>[4x]ADPKCTVSHEVADCSHLKLTQVPDDLPTNITVLNLTHNQLRRLPAANFTRYSQLTSLDVGFNTISKLEPELCQKLPMLKVLNLQHNELSQLSDKTFAFCTNLTELHLMSNSIQKIKNNPFVKQKNLITLDLSHNGLSSTKLGTQVQLENLQELLLSNNKIQALKSEELDIFANSSLKKLELSSNQIKEFSPGCFHAIGRLFGLFLNNVQLGPSLTEKLCLELANTSIRNLSLSNSQLSTTSNTTFLGLKWTNLTMLDLSYNNLNVVGNDSFAWLPQLEYFFLEYNNIQHLFSHSLHGLFNVRYLNLKRSFTKQSISLASLPKIDDFSFQWLKCLEHLNMEDNDIPGIKSNMFTGLINLKYLSLSNSFTSLRTLTNETFVSLAHSPLHILNLTKNKISKIESDAFSWLGHLEVLDLGLNEIGQELTGQEWRGLENIFEIYLSYNKYLQLTRNSFALVPSLQRLMLRRVALKNVD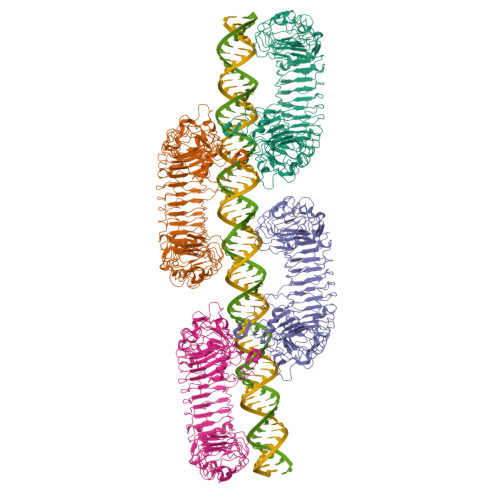SSPSPFQPLRNLTILDLSNNNIANINDDMLEGLEKLEILDLQHNNLARLWKHANPGGPIYFLKGLSHLHILNLESNGFDEIPVEVFKDLFELKIIDLGLNNLNTLPASVFNNQVSLKSLNLQKNLITSVEKKVFGPAFRNLTELDMRFNPFDCTCESIAWFVNWINETHTNIPELSSHYLCNTPPHYHGFPVRLFDTSSCKSGRLVPRGSHHHHHH>[3x]MGSSHHHHHHSQDPENLYFQGTGKFRYMPFSPAGTPFGFTDRRYLTMNEVGYVSTVKNSEQYSITVSFFDVGRFREYHFEDLFGYDLCFLNEKGTLFGQSKTGQIQYRPHDSIHSNWTKIIPLQAGERITSVAATPVRVIVGTSLGYFRSFNQFGVPFAVEKTSPIVALTAQNYRVFSVHYSQFHGLSYSLSELGTSSKRYYKRECPLPMSLPNINSDMKKDANLDYYNFNPMGIKSLFFSSYGDPCIFGSDNTLLLLSKWRSPEESKWLPILDSNMEIWKMSGGKETTDIHVWPLALAYDTLNCILVKGKHIWPEFPLPLPSEMEIRMPVFVKSKLLEENKAILNKKNEIGADTEAEEGEEDKEIQIPVSMAAEEEYLRSKVLSELLTDTLENDGEMYGNENEVLAALNGAYDKALLRLFASACSDQNVEKALSLAHELKQDRALTAAVKISERAELPSLVKKINNIREARYEQQLK;>[3x]SHAKDVKIQETIRKLNRFKPT

Ctf4 forms a homotrimer that has the potential to connect the CMG helicase to one or two Pol α complexes, via the α-helical bundle at the carboxyl terminus of each Ctf4 protomer, which binds to a short conserved motif in the GINS component of CMG and the Pol1 catalytic subunit of Pol α (Simon et al., 2014). Here, we identify new Ctf4 partners in addition to Pol α and helicase, all of which contain a “Ctf4-interacting-peptide” or CIP-box. Crystallographic analysis classifies CIP-boxes into two related groups that target different sites on Ctf4. In addition to its role as a bridge between the CMG helicase and Pol α, our data indicate that Ctf4 functions as a key hub within the replisome, linking the helicase to a diverse set of partners.

Multiple hits of two more new partners of Ctf4 461–927 were also identified in the screen, namely the Dpb2 subunit of Pol ε (Araki et al., 1991) and the rDNA-associated protein Tof2 (Huang et al., 2006, Park and Sternglanz, 1999). As Tof2 had not previously been shown to interact with components of the chromosome replication machinery, we expressed a tagged form of Tof2 in budding yeast cells and found that Tof2 co-purified with Ctf4 in both G1-phase and S phase. This is consistent with direct association of Tof2 with Ctf4, and we confirmed by native mass spectrometry and pull-down assays that a peptide containing the Tof2 CIP-box could indeed bind directly to Ctf4 in vitro. To establish how the divergent Tof2 CIP-box binds to Ctf4, we soaked the corresponding peptide into Ctf4CTD crystals. Remarkably, the peptide bound to a different site to that recognized by the “type I” CIP-boxes of Dna2, Sld5, and Pol1, namely to the side of the C-terminal blade in the β-propeller domain of Ctf4CTD. To validate these findings, we used the crystal structure to generate the ctf4-3E allele, by glutamate mutation of three key hydrophobic residues at the interface between Ctf4 and the Tof2 CIP-box. Critically, the ctf4-3E mutations abolished interaction with full-length Tof2 in the yeast two-hybrid assay, without affecting interaction with Dna2 and Pol1. Conversely, Ctf4-4E (with mutated binding site for type I CIP-boxes) was still able to interact with both Tof2 and Dpb2, despite being unable to interact with Dna2 and Pol1. These findings indicate that both Tof2 and Dpb2 are archetypal “type II CIP-box proteins”, with a distinct binding site on Ctf4 to the type I CIP-boxes of factors such as Dna2, Pol1, and Sld5. However, we found that the size of chromosome 12 was strikingly reduced in both tof2-4A and tof2Δ cells, indicating that tethering of Tof2 to Ctf4 is important during chromosome replication for the preservation of rDNA copy number.>[2x]MSLTRTQTYRATIESDIESYLKKAIPIRAPESVFEPMHHLTFAAPRTSASALCVAACELVGGDRSDAMAAAAAVHLMHVAAYTHENLPLTDGPMSKSEIQHKFDPNIELLTGDGIIPFGLELMARSMDPTRNNPDRILRAIIELTRVMGSEGIVEGQYHELGLNQLNDLELIEYVCKKKE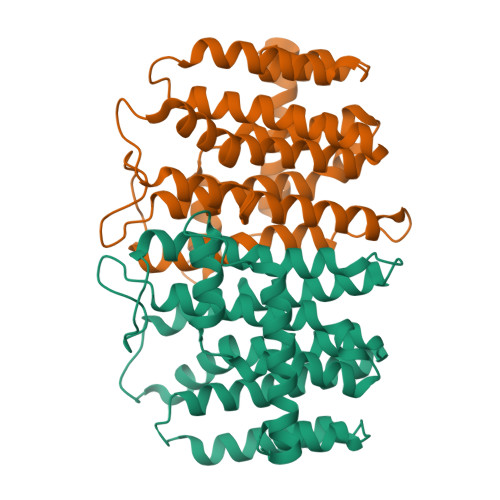GTLHACGAACGAILGGCDEDKIEKLRRFGLYVGTVQGLLGKNRSGFEGRIKELKELAVKELESFGGEKIELIRGVFELEHSLAGVEGHHHHHH>MLLAHISDTHFRSRGEKLYGFIDVNAANADVVSQLNALRERPDAVVVSGDIVNCGRPEEYQVARQILGSLNYPLYLIPGNHDDKALFLEYLQPLCPQLGSDANNMRCAVDDFATRLLFIDSSRAGTSKGWLTDETISWLEAQLFEGGDKPATIFMHHPPLPLGNAQMDPIACENGHRLLALVER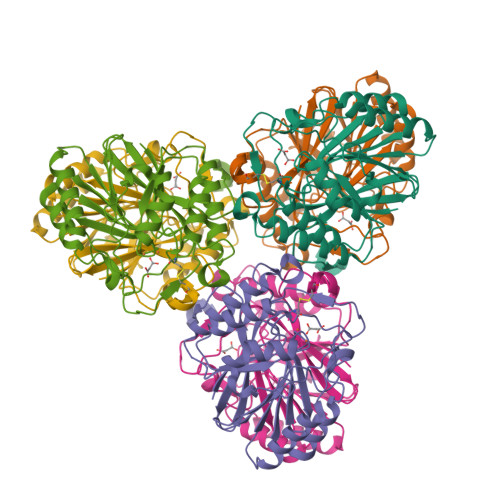FPSLTRIFCGHNHSLTMTQYRQALISTLPGTVHQVPYCHADTDPYYDLSPASCLMHRQVGEQWVSYQHSLAHYAGPWLYDENISCPTEER[2x]> GAMATEEEKKILIPILRKKPVRTISGVAVVAVMTSPAKCPHGKCIFCPGGLDSVFGDVPQSYTGREPATMRGLMFNFDPYLQTRARIEQLEKVGHPTDKIELIIMGGTFPAREIEYQDWFIKRCLDAMNERESKSLEEAQKINETAKHRCVALCIETRPDYCSEKEINQMLKLGATRVELGVQSIYNEILKLCKRGHSVEDTIKATQLLKDSGLKVSYHLMPGMPGSSIEMDKKMFKEIFTNPDFMPDMVKIYPCLVIEGTELYEMWKRGEFKPYREEEAIEVISYAKSIMPKWVRTSRIQRDIPATVIVDGVKKSNLGELVYKYMEKK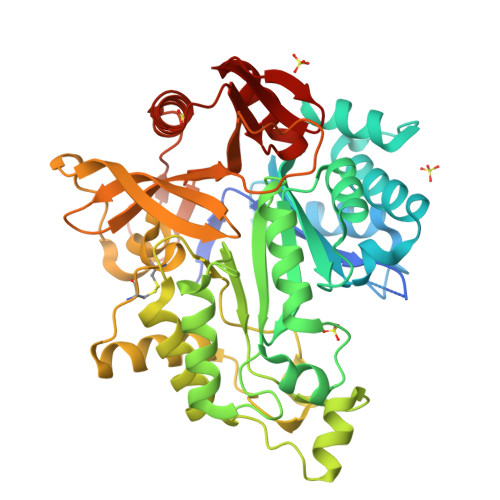GLRCRCIRCREVGHVYYKKGILPDPEHIKLVREDYEASGGTEIFLSFEDVKNDILIAFLRLRDPYKPFRKEIDDKTMLVRQLHVFGWEKALTRDIKEVSWQHMGYGRMLMKEAERIAKEEFGKKKILVTSGIGVREYYRKLGYKRVGAYMGKEL2-(3,4-dihydroxyphenyl)-3,5-dihydroxy-7-methoxy-4H-1-benzopyran-4-one 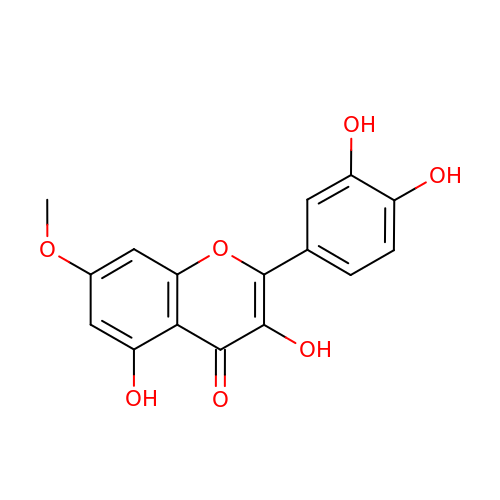| C16 H12 O7 | JGUZGNYPMHHYRK-UHFFFAOYSA-N> 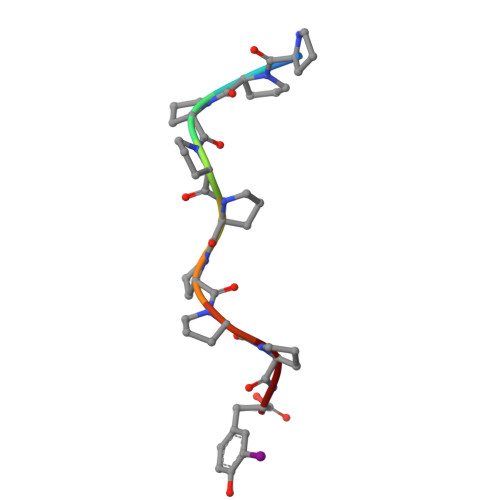PPPPPPPPY> MASAAVANYEEEIVRPVADFSPSLWGDQFLSFSIDNQVAEKYAKEIEALKEQTRNMLLATGMKLADTLNLIDTIERLGISYHFEKEIDDILDQIYNQNSNCNDLCTSALQFRLLRQHGFNISPEIFSKFQDENGKFKESLASDVLGLLNLYEASHVRTHADDILEDALAFSTIHLESAAPHLKSPLREQVTHALEQCLHKGVPRVETRFFISSIYDKEQSKNNVLLRFAKLDFNLLQMLHKQELAQVSRWWKDLDFVTTLPYARDRVVECYFWALGVYFEPQYSQARVMLVKTISMISIVDDTFDAYGTVKELEAYTDAIQRWDINEIDRLPDYMKISYKAILDLYKDYEKELSSAGRSHIVCHAIERMKEVVRNYNVESTWF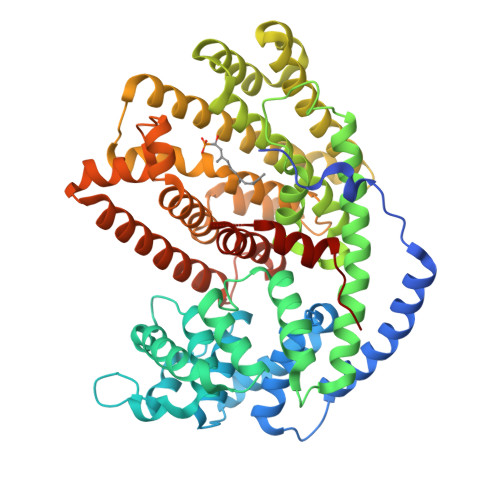IEGYTPPVSEYLSNALATTTYYYLATTSYLGMKSATEQDFEWLSKNPKILEASVIIWRVIDDTATYEVEKSRGQIATGIECCMRDYGISTKEAMAKFQNMAETAWKDINEGLLRPTPVSTEFLTPILNLARIVEVTYIHNLDGYTHPEEVLKPHIINLLVDSIKI>[6x]MPDMKLFAGNATPELAQRIANRLYTSLGDAAVGRFSDGEVSVQINENVRGGDIFIIQSTCAPTNDNLMELVVMVDALRRASAGRITAVIPYFGYARQDRRVRSARVPITAKVVADFLSSVGVDRVLTVDLHAEQIQGFFDVPVDNVFGSPILLEDMLQLNLDNPIVVSPDIGGVVRARAIAKLLNDTDMAIIDKRRPRANVSQVMHIIGDVAGRDCVLVDDMIDTGGTLCKAAEALKERGAKRVFAYATHPIFSGNAANNLRNSVIDEVVVCDTIPLSDEIKSLPNVRTLTLSGMLAEAIRRISNEESISAMFEHHHHHHH

PRPP is synthesized by PRPP synthase (PRPS), which catalyzes the transfer of diphosphate from ATP to ribose-5-phosphate (R5P), thereby generating AMP and PRPP. Class I PRPP synthase is the most widely distributed in phylogeny, including E. coli and humans. Phosphate ion (Pi) is necessary to activate class I PRPS, while ADP, an allosteric inhibitor, competes with Pi and ATP at allosteric and active sites, respectively. In both models, PRPS hexamers are stacked in rows to form filamentous polymers.

Parallel to the two structures, we also solved another type A filament (type AAMP/ADP), which was formed under the conditions of AMP (2 mM)+ADP (2 mM). This structure is almost the same as the former type A filament model, but its allosteric site 2 is bound by AMP rather than ADP. In addition, the allosteric site 1 in type AAMP/ADP model is empty, supporting that the presence of ADP and Pi in the former type A filament model were due to spontaneous hydrolysis of ATP. According to our two type A filament models, the allosteric site 2 of E. coli PRPS may accommodate both AMP and ADP. The type AAMP/ADP filament model suggests that allosteric site 2 may favor AMP over ADP. Our model suggests that AMP/ADP at allosteric site 2 may contribute in the stabilization of the RF loop through the interaction between R102 and α-phosphate of ADP or AMP. Since the stabilization of the RF loop is expected to prevent ADP from entering allosteric site 1 and avoid the interference RF loop on ATP binding, we suspect that AMP/ADP at allosteric site 2 may enhance PRPS activity. The final average resolution of hexamer is estimated to be 2.6 Å.>[2x]IVGGEKALAGECPYQISLQSSSHFCGGTILDEYWILTAAHCVAGQTASKLSIRYNSLKHSLGGEKISVAKIFAHEKYD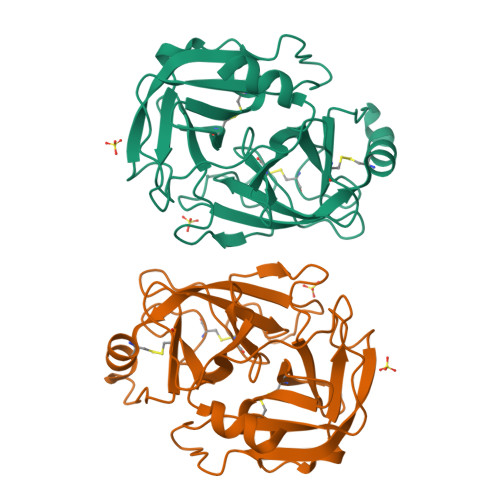SFKIDNDIALIKLKTPMKLDQKNAKAVGLPAKGSDVKVGDQVRVSGWGYLEEGSYSLPSELRRVDIAVVSRKECNELYSKANAEVTDNMICGGDVANGGKDSCQGDSGGPVVDVKNNQVVGIVSWGYGCARKGYPGVYTRVGNFIDWIEIKT2'-5'DIDEOXYURIDINE | C9 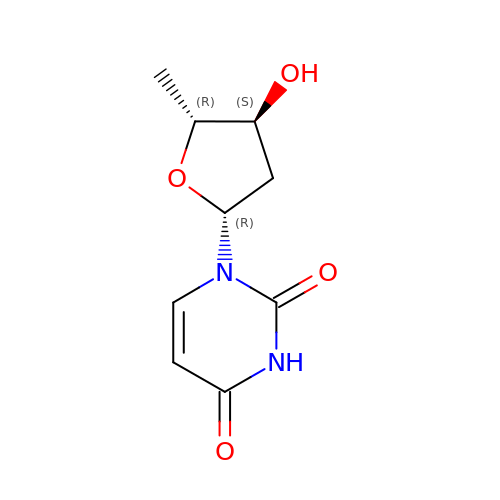H12 N2 O4 | FDCFKLBIAIKUKB-GKROBHDKSA-N>[12x]SGGMKMNPIVELFIKDFTKEVMEENAAIFAGAGLSMSVGYVSWAKLLEPIAQEIGLDVNKENDLVSLAQYYCNENQGNRGRINQIILDEFSRKVDLTENHKILARLPIHTYWTTAYDRLIEKALEEENKIADVKYTVKQLATTKVKRDAVVYKMHGDVEHPSEAVLIKDDYEKYSIKMDPYIKALS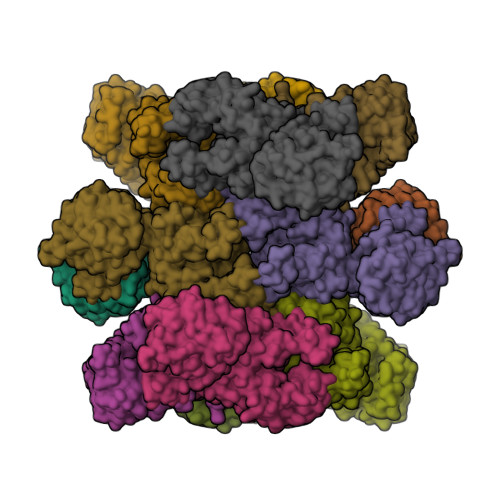GDLVSKTFLFVGFSFTDPNLDYILSRVRSAYERDQRRHYCLIKKEERRPDELEADFEYRVRKQELFISDLSRFNIKTIVLNNYNEITEILQRIENNIKTKTVFLSGSAVEYNHWETEHAEQFIHQLSKELIRKDFNIVSGFGLGVGSFVINGVLEELYMNQGTIDDDRLILRPFPQGKKGEEQWDKYRRDMITRTGVSIFLYGNKIDKGQVVKAKGVQSEFNISFEQNNYVVPVGATGYIAKDLWNKVNEEFETYYPGADARMKKLFGELNNEALSIEELINTIIEFVEILSN> MSGSLSRGNGGKKVLNKNQLLKRNRIRNARSIRAEAVAASSTKTGTPSDLSESGSKLNVDQFISSRQFEVKQLQLAMHNSKAASSTRIFQALPRKLRRRTASHNVRRIPKRMRNRALREMRKSDQQDVLKGSSASSRKAHGLNAKQLYKARMSIKLLRLASKSTSMKLSMPPEVTSSNCHVRQKIKTLKRMIKESSTANPNIKLLNNRMGSYDCTGVNELAPIPKGRVKYTKRQKHFAWLPTHIWNAKRSHMMKRWGYQMVWAPTQKCFKLTHRLGGDTCSSDGALCMDSSYIGTIIVKDKSNDSEGDFLKSIIGKLTAERANLRKYREGQVLFQGLIYSFNEENGEDSTKPLGPCDVFWVQKDTAIIRLHPSIYTQVFNILLQHKEKLTVQDCRYSLASVTLKGAKALESLASCLRSTEYSKSFEQFKMVSMITDHNALPQRCTFAFEAIDPRHLAAPKKLNDSQRKTVNSDDILSLHENYPQDEINAVFNELCDPESRTQSYNNQNTLKEISARRYKLLTATPNSINKTTVPFKESDDPSIPLVIIRRLKTRDWIVVLPWFWLLPLWHLLNRIPRMYHIGLRQFQQIQYENKQLYFPDDYPFTQLGYIENSFYKKEASKTKWDRKPMGKRINFEKIKDIHNTKLPAYSGEIGDFFSSDWRFLQILRNGIDYLQRNDKTLELMDSKKTGQFNAQGVRDINCVNDVLEFCKDYEAKTKAMSLSIEENIPVALCKNRKCQFRTPDSISVNSSSFSLTFFPRCIIAVSCTLLERGHPKDNARIYQVPEKDLEHWLQLAKGVYRPNGRKDHDLKIPLPEVHDLIGFITSGTYHLNCGNGMGIGFIDHHAAIRQPTRYVLIRNVGTNTYRLGEWSKISV;> MSGSLKSLDKKIAKRRQVYKPVLDNPFTNEAHMWPRVHDQPLIWQLLQSSIINKLIHIQSKENYPWELYTDFNEIVQYLSGAHGNSDPVCLFVCNKDPDVPLVLLQQIPLLCYMAPMTVKLVQLPKSAMDTFKSVSKYGMLLLRCDDRVDKKFVSQIQKNVDLLQFPWLNAIKYRPTSVKLLKTTVPIVSKKRQK;> MDRTQTFIKDCLFTKCLEDPEKPFNENRFQDTLLLLPTDGGLTSRLQRQQRKSKLNLDNLQKVSQLESADKQLEKRDYQRINKNSKIALREYINNCKKNTKKCLKLAYENKITDKEDLLHYIEEKHPTIYESLPQYVDFVPMYKELWINYIKELLNITKNLKTFNGSLALLKLSMADYNGALLRVTKSKNKTLIGLQGIVIWDSQKFFIMIVKGNIIDEIKCIPKKGTVFQFEIPISDDDDSALRYSILGDRFKYRSVDRAGRKFKSRRCDDMLYYIQN;> MVRLKSRYILFEIIFPPTDTNVEESVSKADILLSHHRASPADVSIKSILQEIRRSLSLNLGDYGSAKCNSLLQLKYFSNKTSTGIIRCHREDCDLVIMALMLMSKIGDVDGLIVNPVKVSGTIKKIEQFAMRRNSKILNIIKCSQSSHLSDNDFIINDFKKIGRENENENEDD;> MINGVYYNEISRDLDISSSTQCLRFLKETVIPSLANNGNNSTSIQYHGISKNDNIKKSVNKLDKQINMADRSLGLQQVVCIFSYGPHIQKMLSILEIFKKGYIKNNKKIYQWNKLTSFDIKREGRNELQEERLKVPILVTLVSDSEIIDLNLHSFTKQ;> MALKKNTHNKSTKRVTKHPSLKTLTHKQIHTTIFVKSTTPYVSALKRINKFLDSVHKQGSSYVAVLGMGKAVEKTLALGCHFQDQKNKKIEVYTKTIEVLDEVITEGQADIDMESDVEDD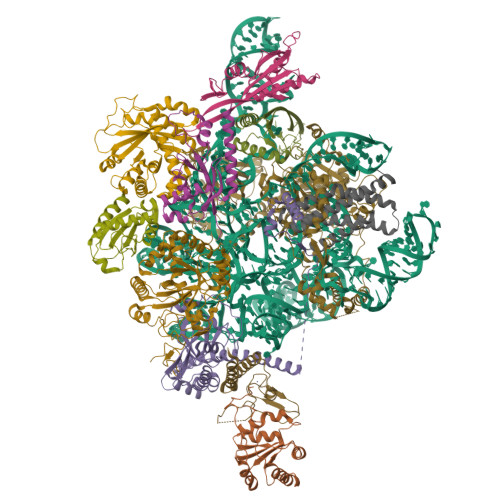DKETQLKKRAVSGVELRIYV;> MGKKTFREWQYFKLSITSFDQDVDDAHAIDQMTWRQWLNNALKRSYGIFGEGVEYSFLHVDDKLAYIRVNHADKDTFSSSISTYISTDELVGSPLTVSILQESSSLRLLEVTDDDRLWLKKVMEEEEQDCKCI;>[2x]MLVDLNVPWPQNSYADKVTSQAVNNLIKTLSTLHMLGYTHIAINFTVNHSEKFPNDVKLLNPIDIKRRFGELMDRTGLKLYSRITLIIDDPSKGQSLSKISQAFDIVAALPISEKGLTLSTTNLDIDLLTFQYGSRLPTFLKHKSICSCVNRGVKLEIVYGYALRDVQARRQFVSNVRSVIRSSRSRGIVIGSGAMSPLECRNILGVTSLIKNLGLPSDRCSKAMGDLASLVLLNGRLRNKSHKQTIVTGGGSGNGDDVVNDVQGIDDVQTIKVVKRSMDAEQLGHASKRHKP;> MNKDQAEKYQERSLRQKYNLLHVLPTLNSRALSGLYYKNFHNSVKRYQIMLPEQLKSGKFCSHCGCVYVPNFNASLQLTTNTEQGDSDELGGESMEGPKKCIQVNCLNCEKSKLFEWKSEFVVPTFGQDVSPMINSTSSGKVSYAVKKPQKSKTSTGKERSKKRKLNSLTNLLSKRNQEKKMEKKKSSSLSLESFMKS;> MDEMDNVIRSLEQEYRLILLLNHRNKNQHRAASWYGSFNEMKRNCGQIITLFSSRRLQAKRLKDVEWVKLHRLLQRALFRQLKRWYWQFNGVIALGQFVTLGCTLVTLLANVRALYMRLWEINETEFIRCGCLIKNLPRTKAKSVVNDVEELGEIIDEDIGNNVQENELVITSIPKPLTENCKKKKKRKKKNKSAIDGIFG> GAQVSTQK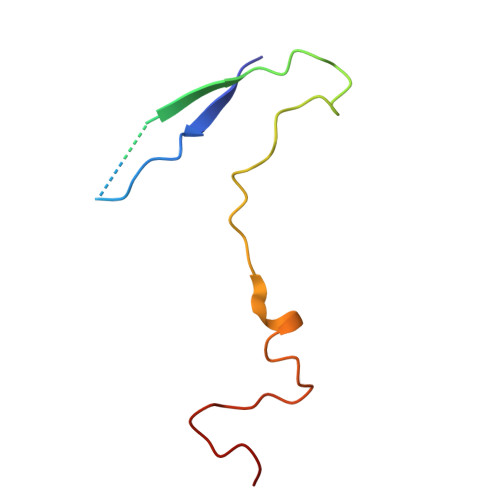TGAHETGLNASGNSIIHYTNINYYKDAASNSATRQDFAQDPGKFTEPVKDIMIKSLPALN>MISVGEIMERANHSLVRMRREGEDLTLEEKAEICSELELQQKYVDIASNIIGDLSSLPIAGKIAGTIAAAAMTATHVASGRLDIEQTLLGCSDLPFDQIKEVLENRFNEIDRKLDSHSAALEEITKLVEKSISVVEKTRKQMNKRFDEVMKSIQDAKVSPIISKINNFARYFDTEKERIRGLKLNDYILKLEEPNGILLHFKESRTPTDDSLQAPLFSIIEEGYAVPKSIDDELAFKVLYALLYGTQTYVSVMFFLLEQYSFLANHYYEKGYLEKYDEYFNSLNNVFLDFKSSLVGTGTSNNEGLLDRVLQVLMTVKNSEFLGLEKNGVDEMLNEKINLFNKIKEEIEGKQKMTLSETPENFAQISFDKDITTPIGDWRDGREVRYAVQYASETLFSKISHWSDPVSVREKACPTLRMPVDQTRRNVLVFRKFDSSKPQLVGEITPYLSNFIDIDRDLYNAASNPDSAVGFKEFTKLNYDGANIRATFDHGRTVFHAAAKSGNDKIMFGLTFLAKSTELNQPDKKGY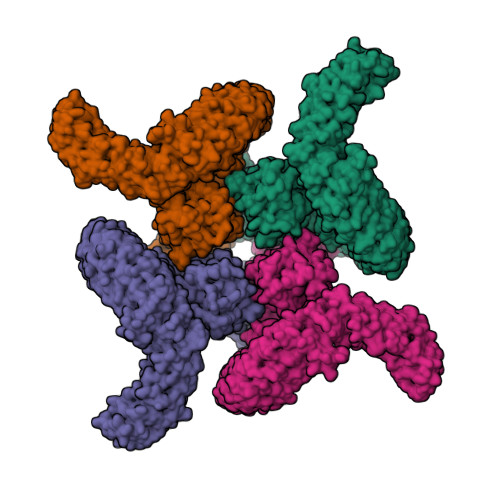TPIHVAADSGNAGIVNLLIQRGVSINSKTYHFLQTPLHLAAQRGFVTTFQRLMESPEININERDKDGFTPLHYAIRGGERILEAFLNQISIDVNAKSNTGLTPFHLAIIKNDWPVASTLLGSKKVDINAVDENNITALHYAAILGYLETTKQLINLKEINANVVSSPGLLSALHYAILYKHDDVASFLMRSSNVNVNLKALGGITPLHLAVIQGRKQILSLMFDIGVNIEQKTDEKYTPLHLAAMSKYPELIQILLDQGSNFEAKTNSGATPLHLATFKGKSQAALILLNNEVNWRDTDENGQMPIHGAAMTGLLDVAQAIISIDATVVDIEDKNSDTPLNLAAQNSHIDVIKYFIDQGADINTRNKKGLAPLLAFSKKGNLDMVKYLFDKNANVYIADNDGMNFFYYAVQNGHLNIVKYAMSEKDKFEWSNTDNNRRDECPNEECAISHFAVCDAVQFDRIEIVKYFVGTLGNFAICGPLHQAARYGHLDIVKYLVEEEFLSVDGSKTDTPLCYASENGHFTVVQYLVSNGAKVNHDCGNGMTAIDKAITKNHLQVVQFLAANGVDFRRKNSRGTTPFLTAVAENALHIAEYLIREKRQDININEQNVDKDTALHLAVYYKNLQMIKLLIKYGIDVTIRNAYDKTALDIAIDAKFSNIVEYLKTKSGKFRREYKSSYGERSLLQTNQISNFIDRKNIEHDHPLFINADNESSELFSKTASNIDVIGTLLLIDVLIRYFSKQGYISKESDSASDGITQAAALSITEKFEDVLNSLHNESAKEQVDLAEVHGKVYAALKSGRNSQIHQILCSSLNSISTLKPEDMEKLESVIMNSHSSVSLPEVTDSANEAYGETLHLFGESCLHSDGILTKKLM[4x]> MAYTTFSQTKNDQLKEPMFFGQPVNVARYDQQKYDIFEKLIEKQLSFFWRPEEVDVSRDRIDYQALPEHEKHIFISNLKYQTLLDSIQGRSPNVALLPLISIPELETWVETWAFSETIHSRSYTHIIRNIVNDPSVVFDDIVTNEQIQKRAEGISSYYDELIEMTSYWHLLGEGTHTVNGKTVTVSLRELKKKLYLCLMSVNALEAIRFYVSFACSFAFAERELMEGNAKIIRLIARDEALHLTGTQHMLNLLRSGADDPEMAEIAEECKQECYDLFVQAAQQEKDWADYLFRDGSMIGLNKDILCQYVEYITNIRMQAVGLDLPFQTRSNP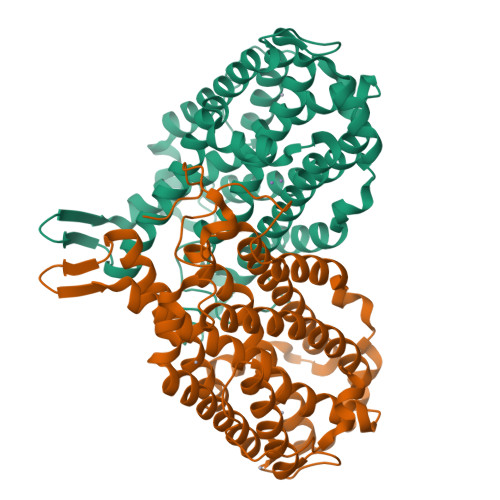IPWINTWL>[2x]GSHMTWLSDFPQAWAETGGMGLAVRQAPLIIPLKATSTPVSIKQYPMSQEARLGIKPHIQRLLDQGILVPCQSPWNTPLLPVKKPGTNDYRPVQDLREVNKRVEDIHPTVPNPYNLLSGLPPSHQWYTVLDLKDAFFCLRLHPT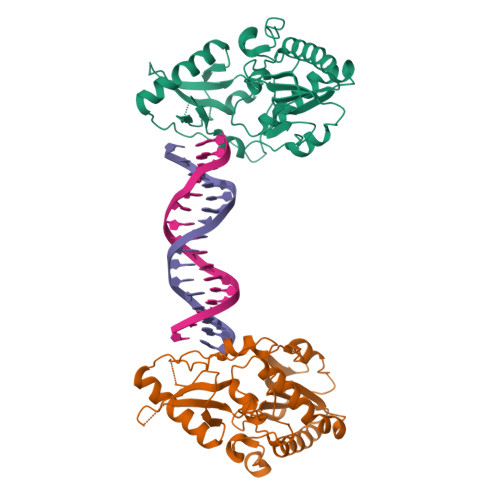SQPLFAFEWRDPEMGISGQLTWTRLPQGFKNSPTLFDEALHRDLADFRIQHPDLILLQYVDDLLLAATSELDCQQGTRALLQTLGNLGYRASAKKAQICQKQVKYLGYLLKEGQR>[6x]MMGPVWRKHYITYRINNYTPDMNREDVDYAIRKAFQVWSNVTPLKFSKINTGMADILVVFARGAHGDDHAFDGKGGIL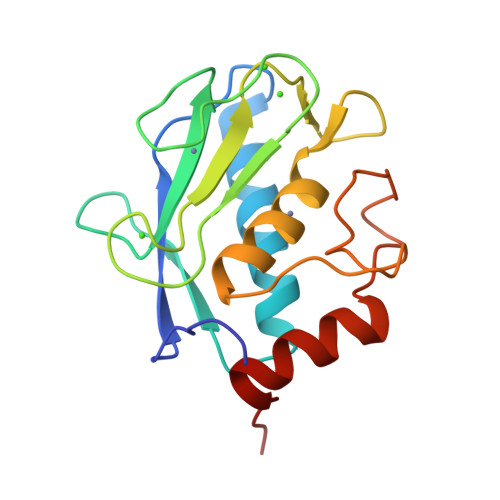AHAFGPGSGIGGDAHFDEDEFWTTHSGGTNLFLTAVHEIGHSLGLGHSSDPKAVMFPTYKYVDINTFRLSADDIRGIQSLYGDPKEN> AEQKTLHIYNWTDYIAPDTVANFEKETGIKVVYDVFDSNEVLEGKLMAGSTGFDLVVPSASYLERQLTAGVFQPLDKSKLPEWKNLDPELLKLVAKHDPDNKFAMPYMWATTGIGYNVDKVKAVLGENAPVDSWDLILKPENLEKLKSCGVSFLDDPEEVFATVLNYLGKDPNSTKADDYTGPATDLLLKLRPNIRYFHSSQYINDLANGDICVAIGWAGSVWQASNRAKEAKNGVNVSFSIPKEGAMAWFDVFAMPADAKNKDEAYQFLNYLLRPDVVAHISDHVFYANANKAATPLVSAEVRENPGIYPPADVRAKLFTQKVQDPKIDRVRTRAWTKVKSGKLEHHHHHH

To gain insight into the evolution and designability of ligand binding and specificity, we analyzed the homologous PBPs, PotF and PotD, which are Escherichia coli putrescine (PUT)-binding protein and spermidine (SPD)-binding protein, respectively. They constitute the first elements of two separate multicomponent uptake systems (PotFGHI and PotABCD) to transport the cationic polyamines PUT and SPD across the cellular membrane. Still, the protein-binding modes differ: PotF shows affinity for PUT and SPD, whereas PotD exclusively binds SPD. Prior to this work, we grafted the seven differences in amino acids from PotD binding pocket onto PotF; this resulted in PotF_SPD, which will be referred to as PotF/D throughout this work to keep naming for mutants more concise.

All prior observations combined led to the following three constructs: the basic double salt bridge reintroduction E39D–Y87S as well as E39D–F88A and E39D–Y87S–F88Y. The removal of this Phe should allow Tyr to flip inside the binding pocket to accommodate PotD-like positioning. We also introduced F88Y in the basic double salt bridge mutant (E39D + Y87S), thereby hijacking a bulky aromatic residue that already points toward the binding pocket to introduce a distal PotD-like Tyr. The highest affinity was measured for the double salt bridge mutant containing the additional F88Y (KD(SPD) ≈ 5.3 μM). To our surprise, all solved structures adopt a PotF/D-like semiclosed conformation. Also, SPD adopts similar positions to the one in PotF/D in all structures. In the highest affinity F88Y mutant, the newly introduced Tyr slightly rotates inside the binding pocket but does not directly interact with the ligand. It is involved in cation–π interactions with R91 and can stack with N65. The second salt bridge residue E184 interacts with D182. Whether all these constructs can completely close in solution remains elusive.>STAGKVIKCKAAVLWEEKKPFSIEEVEVAPPKAHEVRIKMVATGICRSDDHVVSGTLVTPLPVIAGHEAAGIVESIGEGVTTVRPGDKVIPLFTPQCGKCRVCKHPEGNFCLKNDLSMPRGTMQDGTSRFTCRGKPIHHFLGTSTFSQYTVVDEISVAKIDAASPLEKVCLIGCGFSTGYGSAVKVAKVTQGSTCAVFGLGGVGLSVIMGCKAAGAARIIGVDINKDKFAKAKEVGATECVNPQDYKKPIQEVLTEMSNGGVDFSFEVIGRLDTMVTALSCCQEAYGVSVITGVPPDSQNLSMNPMLLLSGRTWKGAIFGGFKSKDSVPKLVADFMAKKFALDPLITHVLPFEKINEGF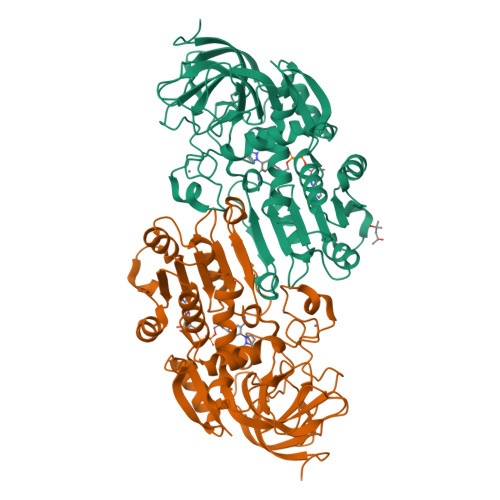DLLRSGESIRTILTF[2x]>[4x]MSLNTSIYGLIGEKLGHSHSSYIHKLIFEKVGIKGIYNLFEVPKEKLKESVDTFKIIKCGGLNVTIPYKVEVMKELYEISEKARKIGAVNTLKFSREGISGFNTDYIGFGKMLSKFRVEIKNNICVVLGSGGAARAVLQYLKDNFAKDIYVVTRNPEKTSEIYGEFKVISYDELSNLKGDVI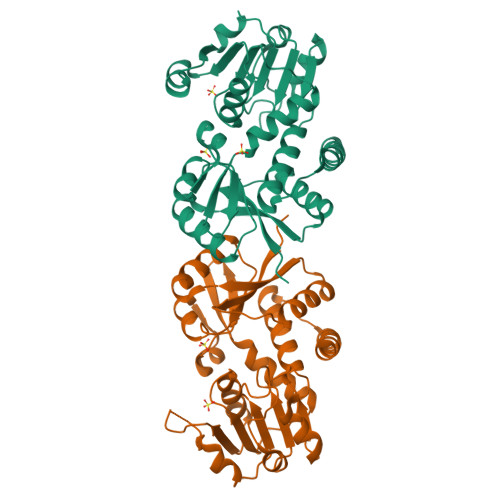INCTPKGMYPKEGESPVDKEVVAKFSSAVDLIYNPVETLFLKYARESGVKAVNGLYMLVSQAAASEEIWNDISIDEIIVDEIFEVLEEKIKSEGHHHHHH In this work we have identified a rice histone demethylase, namely JMJ703, which specifically demethylates methylated histone H3 lysine 4. Our results demonstrate that JMJ703 is essential for plant cell division and stem elongation and specifically demethylates mono-, di-, and trimethylated H3K4 in vivo and in vitro. Finally, the fragment spanning amino acids 139 to 498 (termed c-JMJ703), covering the JmjN and JmjC domains, was deemed to be suitable for crystallographic investigation. The c-JMJ703 molecule presented a canonical overall folding of JMJD2 proteins and contained four of the five domains defined in the structure of c-JMJD2A: the JmjN domain (A139-K199), the long β-hairpin (D200-T271), the mixed domain (L272-V377) and the JmjC domain (L378-A498).

The high resolution structure of the catalytic core of JMJ703 (c-JMJ703) in complex with cofactors and substrate peptide reveals that the overall folding of c-JMJ703 is similar to those defined in animal and yeast JMJD2 that are H3K9 and H3K36 demethylases. The final model was best at a resolution of 2.35 Å with a final Rwork value of 19.3% (Rfree = 22.5%). The electron density indicated the presence of substrate peptide in the c-JMJ703-NOG-H3K4me3 complex. Three of the ten residues in the H3K4me3 peptide (ARTKme3QTARKS) were visible in the c-JMJ703-NOG-H3K4me3 complex structure. This complex structure provided a view of the substrate peptide-binding mode of an H3K4 demethylase. Compared with the structure of c-JMJD2A in complex with methylated H3K9/H3K36 peptide, the methylated H3K4 and its two flanking residues adopted a different binding conformation to c-JMJ703. The methyl groups could not be defined properly in the c-JMJ703-NOG-H3K4me3 complex structure because of low occupancy as indicated by obviously higher B-factor for atoms in H3K4me3 peptide. Fe(II) also interacted with the C-1 carboxyl and C-2 oxo groups of NOG. In the crystal structure of c-JMJ703-NOG-H3K4me3, NOG formed three hydrogen bonds with the side chains of N404 and K412 similar to the JMJD2 homologues. Moreover, NOG interacted indirectly with N490 through two water molecules, a finding that is not observed in mammalian and yeast homologues.

> AKWNPAGARRPVLDEAPVFYPTEEEFEDTLKYIESIRPMAEPYGICRIVPPSSWKPPCLLKDKSIWEGSKFSTRVQKVDKLQNRKSSKKGRRGGMMKRRKLAESEENSATAHTQTGMQQSPERFGFEPGPEFTLQTFQKYADDFSKQYFRKDTSMDSVPSVEDIEGEYWRIVEVPTEEIEVIYGADLETGTFGSGFPKLSPETKSDAEDKYAQSGWNLNNLPRLQGSVLSFEGGDISGVLVPWVYVGMCFSSFCWHVEDHHLYSLNYMHWGAPKLWYGVPGKDAVNLESAMRKHLPELFEEQPDLLHNLVTQFSPSLLKSEGVHVYRCVQHEGEFVLTFPRAYHAGFNCGFNCAEAVNVA;> TKQ> PGPPQGPPQPVQQSKRLQQTQAQVEEVVDIMRVNVDKVLERDSKISELDDRADALQAGASQFEASAGKLKRKFW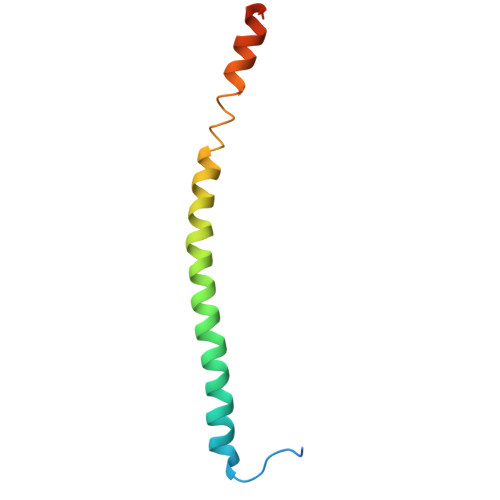WKNCKM> GPLEDYDDEEFLRYLWREYLHPKEYEWVLIAGYIIVFVVALIGNVLVCVAVWKNHHMRTVTNYFIVNLSLAAVLVTITCLPATLVVDITETWFFGQSLCKVIPYLQTVSVSVSVWTLSAIALDRWYAICHPLMFKSTAKRARNSIVIIWIVSCIIM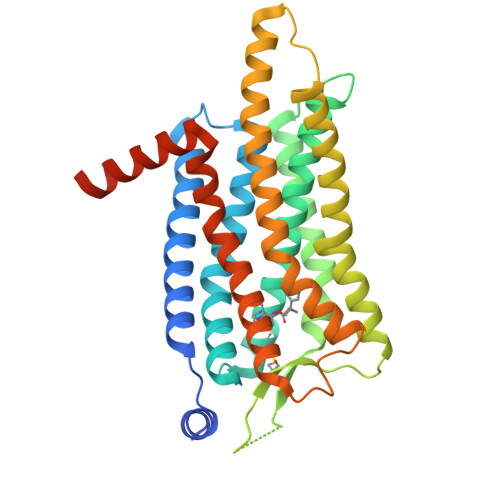IPQAIVMECSTVFPGLAQKTTLFTVCDERWGGEIYPKMYHICFFLVTYMAPLCLMVLAYLQIFRKLWCRQIPGVAAEIKQIRARRKTARMLMIVLLVFAICYLPISILNVLKRVFGMFAHTEDRETVYAWFTFSHWLVYANSAANPIIYNFLSGKFREEFKAAFSCCCLGVHHRQEDRLLEVLFQ dicarbonimidic 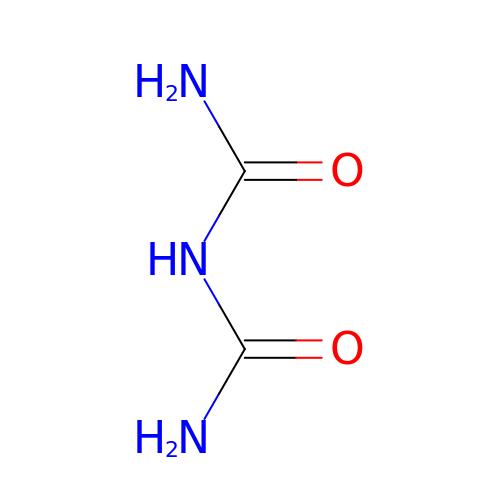diamide | C2 H5 N3 O2 | OHJMTUPIZMNBFR-UHFFFAOYSA-N> GVDTHWFHRNPLKATAPVSFNYYGVVTGPSASKICNDLRSSRARLLELFTDLSCNPEMMKNAADSYFSLLQGFINSLDESTQESKLRYIQNFKWTDTLQGQVPSAQQDAVFELISMGFNVALWYTKYASRLAGKENITEDEAKEVHRSLKIAAGIFKHLKESHLPKLITPAEKGRDLESRLIEAYVIQCQAEAQEVTIARAIELKHAPGLIAALAYETANFYQKADHTLSSLEPAYSAKWRKYLHLKMCFYTAYAYCYHGETLLASDKCGEAIRSLQEAEKLYAKAEALCKEYGETKGPGPTVKPSGHLFFRKLGNLVKNTLEKCQRENGFIYFQKIPTEAPQLELKANYGLVEPIPFEFP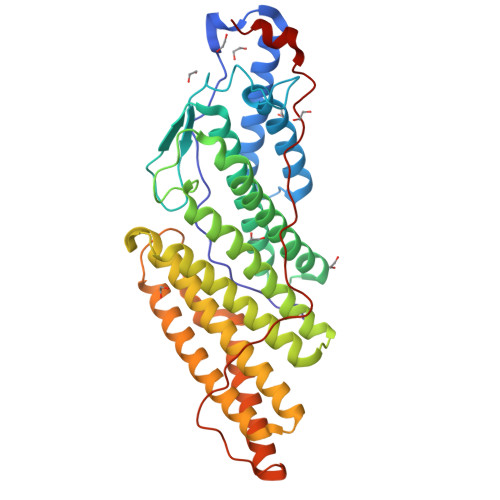PTSVQWTPETLAAFD> MEPLYDKNGAVLFGEPSDTH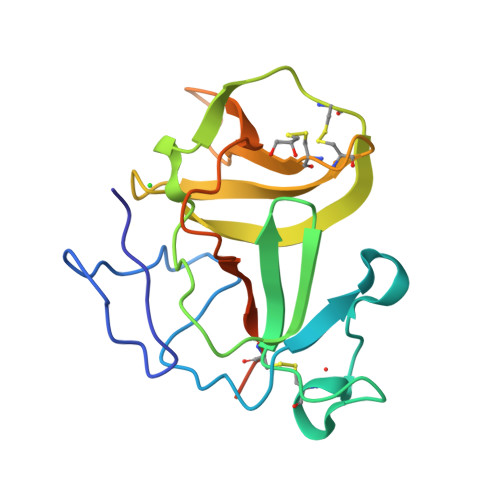PQSTLKLPHPRGEKEVIVGIRDLPRKGDCRTGNRLGPVSGLFVKPGPVFYQDYSGPVYHRAPLEQFKQAPMCEVTKRIGRVTGSDGNLYHMYVCTDGCILVKTAKREGQDVLKWVYNVLDSPIWVTSCPVDKLAAALEHHHHHH> MSKSKVDNQFYSVEVGDSTFTVLKRYQNLKPIGSGAQGIVCAAYDAVLDRNVAIKKLSRPFQNQTHAKRAYRELVLMKCVNHKNIISLLNVFTP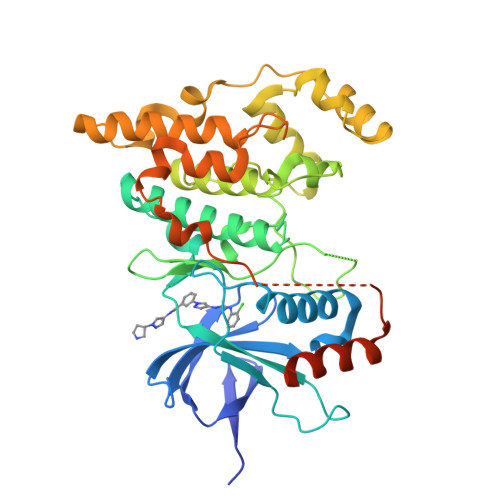QKTLEEFQDVYLVMELMDANLCQVIQMELDHERMSYLLYQMLCGIKHLHSAGIIHRDLKPSNIVVKSDCTLKILDFGLARTAGTSFMMTPYVVTRYYRAPEVILGMGYKENVDIWSVGCIMGEMVRHKILFPGRDYIDQWNKVIEQLGTPCPEFMKKLQPTVRNYVENRPKYAGLTFPKLFPDSLFPADSEHNKLKASQARDLLSKMLVIDPAKRISVDDALQHPYINVWYDPAEVEAPPPQIYDKQLDEREHTIEEWKELIYKEVMNSEEKTKNGVVKGQPSPSGAAVNS> SMTIQEIIQQRNIRSLFHFTHSDNLTSILDNGLMSRSELDNENNEYNCNDEERIDGHPDAICLSVSYPNAKMFYKYRCLKPGDWVILEINPSVLWAKDCAFYPTNAASNNVRFINLDLMKGAEAFSALFSENVFGIQRDVNLPSEYTTDV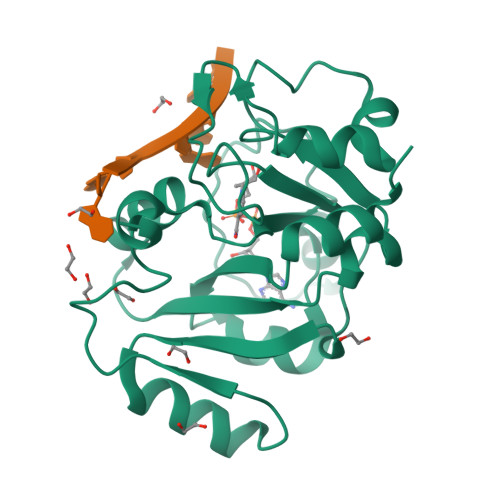QAAILVFEKIPPSYIISTFHPNKESAEHFKRLYPQTIQRYYDNLNARTLYSQRHYYLG4-nitro-2-({4-[3-(trifluoromethyl)phenyl]piperazin-1-yl}methyl)phenol | C18 H18 F3 N3 O3 | 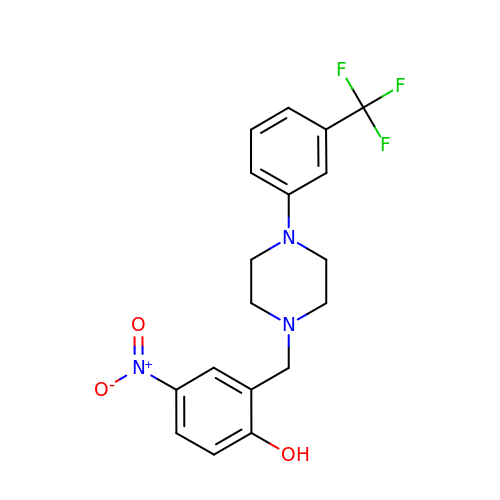NZPUDXBEGUWKPV-UHFFFAOYSA-N>[2x]MKMNQFINALMAKMTLDEKIGQLNLPGAGDITTGQASSSGIAQKIKEGKVGGLFNIKSVTKIKEVQRIAVEESRLKIPLLFGMDVIHGYETAFPIPLGLSCTWDMELIEKSARIAAIEASADGICWTFSPMVDISRDPRWGRVSEGSGEDPYLGAQIAKAMVKGYQGKDFSDNTSIMACVKHFALYGAGEAGRDYNTVDMSRVRMYNEYFPPYKAAVDAGVGSVMTSFNEIDGIPATGNKWLMTDVLRKRIGAFKGFVVTDYTAINEMIDHGMGDLQTVSALALRAGVDMDMVGEGFLTTLKKSLQEGKITQAQIDAACKRILEAKYKLGLFSDPYKYCNEERARTQIFTPEHRKIAREIAAQSFVLLKNDNNVLPLKKSGTIALVGPLADNRVNMPGTWSVAAKHAESVSLLEGLKKAAGNDARILYAHGSNLDEDKSLIERATMFGKTLKYDPRPKDVVIK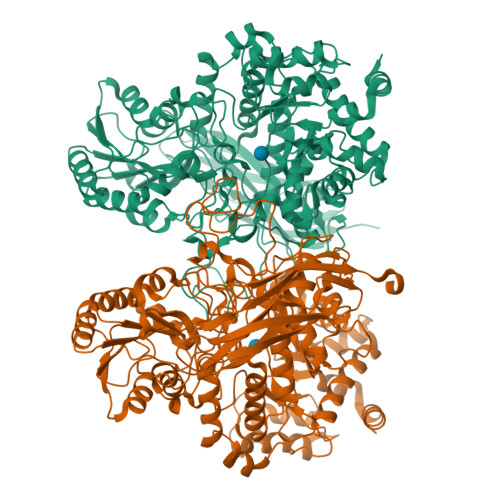EAVDIANQADVIVAALGESAEMSGEASSRSNIEIPALQRELLQALLKTGKPVVLVLFTGRPLALTWEHENVPAILNVWFAGTEAGDAISDALFGVVNPSGKLSATFPRNVGQVPIYYNHKNTGRPLPEGQWFQKFRSNYLDVPNDPLYPFGYGLSFTKFTYGDLKLSSTNLKGNQTLTASIELTNSGDYDGAEVVQLYIRDLVGSTTRPVKELKGFQKVFLKKGETKTITFKITPEDLKFYNYDLKYDWEPGEFVIMVGGNSRDLKSQKINWLKDPAFLYKVVINSKLEGKPIPNPLLGLDSTRTGHHHHHH Protein ADP-ribosylation is a highly dynamic post-translational modification. The rapid turnover is achieved, among others, by ADP-(ribosyl)hydrolases (ARHs), an ancient family of enzymes that reverses this modification. Reversal of the bulk of PAR modification is mediated by poly(ADP-ribosyl)glycohydrolase (PARG) converting the polymer chain to a mono(ADP-ribosyl) (MAR) modification (Lin et al., 1997, Slade et al., 2011). For example, linkages to glutamate/aspartate are hydrolyzed by macrodomain proteins (Jankevicius et al., 2013, Rosenthal et al., 2013, Sharifi et al., 2013), whereas linkages to arginine and serine are cleaved by ARH1 and ARH3, respectively, two members of the structurally unrelated (ADP-ribosyl)hydrolases (ARHs) family (Fontana et al., 2017, Moss et al., 1988).

In order to probe whether the differences between the active sites have an effect on substrate recognition, we used the ADPr analogues adenosine diphosphate (hydroxymethyl)pyrrolidinediol (ADP-HPD) and -monoalcohol (ADP-HPM). These compounds were originally designed as PARG inhibitors and contain pyrrolidine instead of the distal ribose as well as differing in the number of hydroxyl substituents. In order to elucidate further the selectivity of these inhibitors, we performed crystallization experiments with hARH1 and LchARH3 in the presence of these ligands and solved the structures of the hARH1:ADP-HPM, LchARH3:ADP-HPD, and LchARH3:ADP-HPM complexes. In contrast, the orientation of ADP-HPD in the active site is similar to ADPr. The only differences are that the 2″ OH moiety of ADP-HPD is bridging MgI and MgII and a flip of C5″ rotates the pyrrolidine ring slightly away from the Mg2+ ions allowing for a more relaxed conformation. However, the 1″ OH in the LchARH3:ADPr complex appears to take part in the second coordination sphere of MgII, whereas this is not the case in the hARH1:ADPr complex. In the latter, the ADPr takes on a more relaxed conformation, which is mimicked in the LchARH3:Arg-ADPr and :ADP-HPD complexes, thus suggesting that an α-linked oxygen draws the ribose ring closer to the magnesium ion. In our structures, this moiety is either coordinating MgI (ADPr structure) or bridging between the Mg2+ ions (ADP-HPD, Arg-ADPr, and IDPr). In line with the previous results, hARH3 is most efficiently inhibited by ADP-HPD and to a lesser extent by ADPr and ADP-HPM (IC50 of 0.587 μM, 3.2 μM, and 480 μM, respectively). (2) Comparison of the potency of ADP-HPD and -HPM as ARH3 inhibitors as well as our differential scanning fluorimetry (DSF) data suggests that the stabilization of the binuclear metal center could increase the efficiency of inhibitors.

>GPMVSLAQVRGALCGALLGDCMGAEFEGSDAVELPDVLEFVRLLEKEKKAGTLFYTDDTAMTRAVIQSLIAKPDFDEVDMAKRFAEEYKKEPTRGYGAGVVQVFKKLLSPKYSDVFQPAREQFDGKGSYGNGGAMRVASIALAYPNIQDVIKFARRSAQLTHASPLGYNGAILQALAVHFALQGELKRDTFLEQLIGEMERIEGGEMSASDAGEHDRPNEVKLPFCSRLKKIKEFLASSNVPKADIVDELGHGIAALESVPTAIYSFLHCMESDPDIPDLYNNLQRTIIYSISLGGDTDTIATMAGAIAGAYYGMDQVTPSWKRSCEAIVETEESAVKLYELYCKQLKTP[2x]>NFNSQNGVNKDEKDHLIERLYREISGLKAQLENMKTESQRVVLQLKGHVSELEADLAEQQHLRQQAADDCEFLRAELDELRRQREDTEKAQRSLSEIERKAQANEQRYSKLKEKYSELVQ[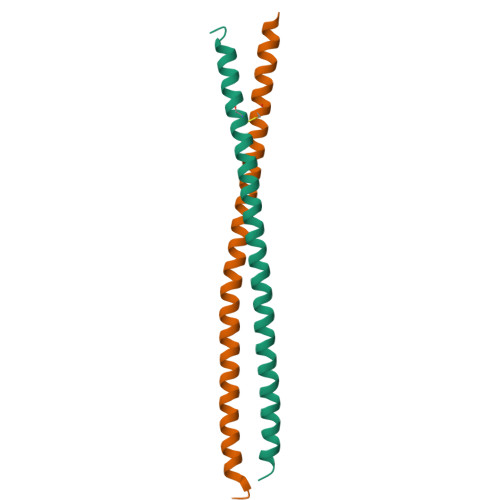2x]> MSTYYFVIVGQNDNPIYEKEFSTVNKELRKED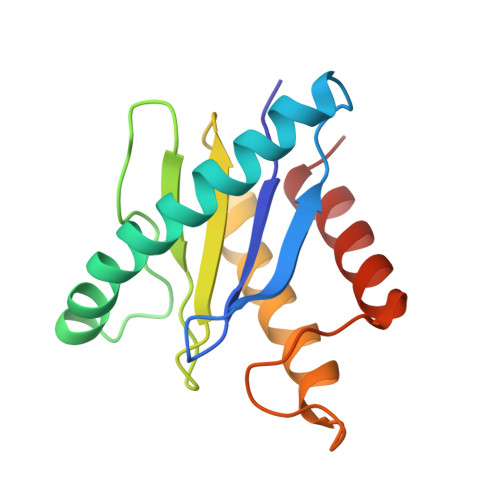HRHLTQFIAHAALDLVDEHKWKTANMQLKSIDRFNQWFVSAFITASQIRFIIVHDNKNDEGIKNFFNEMYDTYIKNSMNAFYRINTPIKSPMFEKKSEIFGRKYLLS>[2x]GSSHHHHHHSSGLVPRGSMS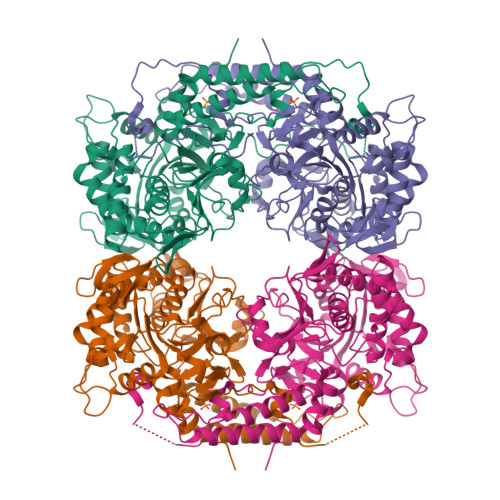TSWSDRLQNAADMPANMDKHALKKYRREAYHRVFVNRSLAMEKIKCFGFNMDYTLAVYKSPEYESLGFELTVERLVSIGYPQELLSFAYDSTFPTRGLVFDTLYGNLLKVDAYGNLLVCAHGFNFIRGPETREQYPNKFIQRDDTERFYILNTLFNLPETYLLACLVDFFTNCPRYTSCETGFKDGDLFMSYRSMFQDVRDAVDWVHYKGSLKEKTVENLEKYVVKDGKLPLLLSRMKEVGKVFLATNSDYKYTDKIMTYLFDFPHGPKPGSSHRPWQSYFDLILVDARKPLFFGEGTVLRQVDTKTGKLKIGTYTGPLQHGIVYSGGSSDTICDLLGAKGKDILYIGDHIFGDILKSKKRQGWQTFLVIPELAQELHVWTDKSSLFEELQSLDIFLAELYKHLDSSSNERPDISSIQRRIKKVTHDMDMCYGMMGSLFRSGSRQTLFASQVMRYADLYAASFINLLYYPFSYLFRAAHVLMPHESTVEHTHVDINEMESPLATRNRTSVDFKDTDYKRHQLTRSISEIKPPNLFPLAPQEITHCHDEDDDEEEEEEEE> MGKRL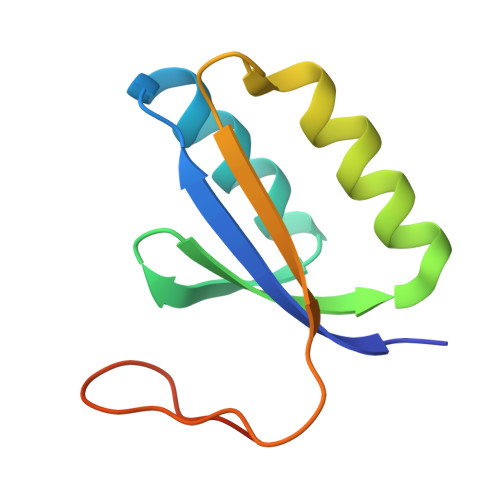YAVAYDIPDDTRRVKLANLLKSYGERVQLSVFECYLDERLLEDLRRRARRLLDLGQDALRIYPVAGQVEVLGVGPLPELREVQVL> GPLGSSQIPAS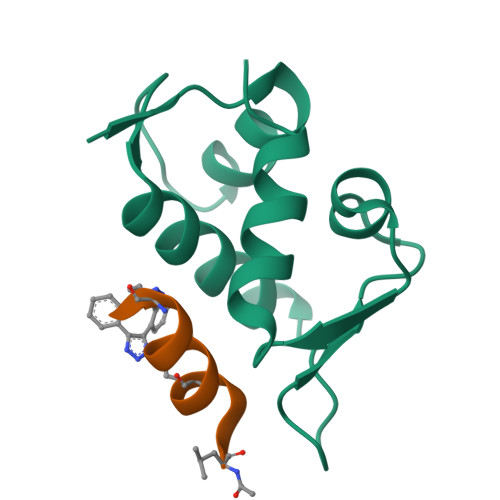EQETLVRPKPLLLKLLKSVGAQKDTYTMKEVLFYLGQYIMTKRLYDAAQQHIVYCSNDLLGDLFGVPSFSVKEHRKIYTMIYRNLV;> LTFAEYWAQLAS> GSSVPAYSGWTLVWADDFTGPAGSLPSSENWIFDTGHSYPGGPDNWGTGEIQRYTDDPANVSLDGNGNLRITPLRSASGEWTSARIETRRADFKPAPGGVLRIEARIQLPNVTGEAALGYWPAFWALGSPYRGDYWNWPRIGE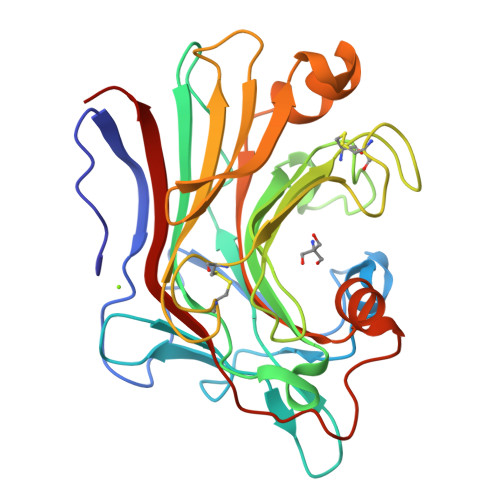FDIMENVNGLNRVWGVLHCGVAPGGPCNEYDGLGNSRECPGTTCQAGMHTYRFEWDTSRSPNELRWYVDGQHYHTIRQDQLDATTWSNMTGHGGYFLLLNVAMGGAFPDGVAGHATPTSATVPGRSMIVDYVGVWQSGGD>[3x]MGSSHHHHHHSSGPQQGLRSNSDDAEKPVVPVPTGDVAIYTTTSSLTRDLTRDAVNFSPKDNLAPTTITLNPAEQYQTMDGFGAAITGSTCYNLLLMKPADRHAFLTETFSDKDGFGFSYIRISIGCSDFSLSEYTCCDTKGIENFALQSEEKDYILPILKEILAINPSIKVIAAPWTCPKWMKVKSLTDRTPLDSWTNGQLNPDYYQDYATYFVKWIQAFKAEGIDIYAVTPQNEPLNRGNSASLYMEWEEQRDFVKTALGPQMKAAGLSTKIYAFDHNYNYDNIESQKNYPGKIYEDAAASQYLAGAAYHNYGGNREELLNIHQAYPEKELLFTETSIGTWNSGRDLSKRLMEDMEEVALGTINNWCKGVIVWNLMLDNDRGPNREGGCQTCYGAVDINNSDYKTIIRNSHYYIIAHLSSVVKPGAVRIATTGYTDNGITCSAFENTDGTYAFVLINNNEKSKKITVSDGQRHFAYDVPGKSVTSYRWAKSK

Our data show that this locus orchestrates the degradation of 1,6-β-glucan, and this enables B. thetaiotaomicron to utilize this fungal polysaccharide. The critical enzyme encoded by the PUL is BT3312, an endo-1,6-β-glucanase that is displayed on the bacterial surface, allowing direct access to the intact glycan. The enzyme showed no activity on 1,3-β-glucan, 1,4-β-glucan, or 1,6-β-galactan but was active on the 1,6-β-glucan pustulan, producing a range of oligosaccharides in the initial phases of the degradative process. The crystal structure of the endo-1,6-β-glucanase shows that substrate recognition is mediated by shape complementarity of the substrate-binding cleft and the hooked U-shaped conformation of 1,6-β-glucan, rather than through extensive hydrogen-bonding interactions with the polysaccharide.

The crystal structure revealed that BT3312 comprises two domains. The catalytic domain adopts a (β/α)8 barrel fold (TIM barrel), extending from residues Asp82 to Lys427, and a β-sandwich domain comprising sequences from both the N and C termini. The TIM barrel contains a central eight-stranded β-barrel, and extending from each β-strand is an α-helix. Extended loops link the α-helices with the β-barrel, and a small β-sheet comprising three anti-parallel strands is inserted into the loop connecting β-strand-8 and α-helix-8. The β-sandwich domain contains seven antiparallel β-strands in one sheet, with two contributed by the N-terminal region of the enzyme. Based on analysis of other clan GH-A members, the substrate-binding site of BT3312 is predicted to be positioned on top of the β-barrel. Inspection of this region of the enzyme reveals a deep U-shaped cleft that houses the catalytic residues. The active site cleft of BT3312 adopts a different topology to the substrate-binding regions of other GH-A endo-acting enzymes, which typically display linear or curved clefts that are open at both ends. Interestingly, NMR analysis of Candida glabrata 1,6-β-glucan revealed a hooked, U-shaped conformation, which is complementary to the topology of the substrate-binding region of BT3312 (see below). Thus, the candidate catalytic residues are Glu238 (acid/base) and Glu339 (nucleophile).Cation-chloride cotransporters (CCC) are central to the regulation of intracellular Cl− concentration and have key physiological roles in neuronal excitability, trans-epithelial salt and water movement, and regulation of cell volume. The CCCs are strictly electroneutral transporters, NKCCs transporting two Cl− ions coupled to the movement of one Na+ and one K+, whereas NCC and KCC couple the movement of one Cl− ion and either Na+ or K+ respectively. All CCCs are feedback-regulated by the concentration of intracellular Cl−—this is mediated by the WNK (kinase with no lysine)-SPAK/OSR1 (SPS1-related proline/alanine-rich kinase/oxidative stress-responsive kinase 1) signaling pathway. Here, using single-particle cryo-electron microscopy (cryo-EM), we report the structures of human NKCC1 (hNKCC1a) and mouse KCC2 (mKCC2a) at 3.5 and 3.8 Å resolution, respectively.

The final model of hNKCC1 was primarily focused on the transmembrane and extracellular regions from the high-resolution map, although we were also able to determine the overall structure of hNKCC1 including the dimeric C termini from a medium resolution map. We have strong evidence that both of our structures represent inactive states. In the case of hNKCC1, we analyzed phosphorylation of the N terminus using a phospho-specific antibody—as shown in Supplementary Fig. 6a, there is no detectable phosphorylation of the protein as prepared for cryo-EM, and from extensive previous reports, we, therefore, know that this protein must be inactive. Like in DrNKCC140 and hKCC139, we note densities within the cleft at the dimer interface and we attribute these to four lipid molecules with lipid tails in the hydrophobic cavity contributed by TM residues, and hydrophilic heads facing intracellularly. In our inward-open structure of hNKCC1, extracellular access to the pore is blocked by the side chain carbonyl of E389 from TM3 interacting with the side chain amino group of R307 of TM1b and by L671 from TM10 —the narrowest open radius of this potential “gate” is ~1 Å. To test the importance of these residues we examined the transport activity of hNKCC1 mutants. Mutation of any of these residues resulted in Cl− transport activity that is <20% of wild-type activity, with changes in R307 and E389 being particularly impactful; on the other hand, mutagenesis of neighboring E670 has little effect on function. At the intracellular end of the inward-open pore, it is noteworthy that R358 from ICL1 interacts with D632 from adjacent TM8. The most populated Na+ binding site is defined by backbone carbonyls including L297, W300 in TM1, A610 in TM8, and hydroxyl oxygen atoms of S613 and S614 in TM8 —this site (S1) accounts for 40.6% of TM domain Na+ binding sites in the simulation data.

>MEPRPTAPSSGAPGLAGVGETPSAAALAAARVELPGTAVPSVPEDAAPASRDGGGVRDEGPAAAGDGLGRPLGPTPSQSRFQVDLVSENAGRAAAAAAAAAAAAAAAGAGAGAKQTPADGEASGESEPAKGSEEAKGRFRVNFVDPAASSSAEDSLSDAAGVGVDGPNVSFQNGGDTVLSEGSSLHSGGGGGSGHHQHYYYDTHTNTYYLRTFGHNTMDAVPRIDHYRHTAAQLGEKLLRPSLAELHDELEKEPFEDGFANGEESTPTRDAVVTYTAESKGVVKFGWIKGVLVRCMLNIWGVMLFIRLSWIVGQAGIGLSVLVIMMATVVTTITGLSTSAIATNGFVRGGGAYYLISRSLGPEFGGAIGLIFAFANAVAVAMYVVGFAETVVELLKEHSILMIDEINDIRIIGAITVVILLGISVAGMEWEAKAQIVLLVILLLAIGDFVIGTFIPLESKKPKGFFGYKSEIFNENFGPDFREEETFFSVFAIFFPAATGILAGANISGDLADPQSAIPKGTLLAILITTLVYVGIAVSVGSCVVRDATGNVNDTIVTELTNCTSAACKLNFDFSSCESSPCSYGLMNNFQVMSMVSGFTPLISAGIFSATLSSALASLVSAPKIFQALCKDNIYPAFQMFAKGYGKNNEPLRGYILTFLIALGFILIAELNVIAPIISNFFLASYALINFSVFHASLAKSPGWRPAFKYYNMWISLLGAILCCIVMFVINWWAALLTYVIVLGLYIYVTYKKPDVNWGSSTQALTYLNALQHSIRLSGVEDHVKNFRPQCLVMTGAPNSRPALLHLVHDFTKNVGLMICGHVHMGPRRQAMKEMSIDQAKYQRWLIKNKMKAFYAPVHADDLREGAQYLMQAAGLGRMKPNTLVLGFKKDWLQADMRDVDMYINLFHDAFDIQYGVVVIRLKEGLDISHLQGQEELLSSQEKSPGTKDVVVSVEYSKKSDLDTSKPLSEKPITHKVEEEDGKTATQPLLKKESKGPIVPLNVADQKLLEASTQFQKKQGKNTIDVWWLFDDGGLTLLIPYLLTTKKKWKDCKIRVFIGGKINRIDHDRRAMATLLSKFRIDFSDIMVLGDINTKPKKENIIAFEEIIEPYRLHEDDKEQDIADKMKEDEPWRITDNELELYKTKTYRQIRLNELLKEHSSTANIIVMSLPVARKGAVSSALYMAWLEALSKDLPPILLVRGNHQSVLTFYS[2x]> IIGG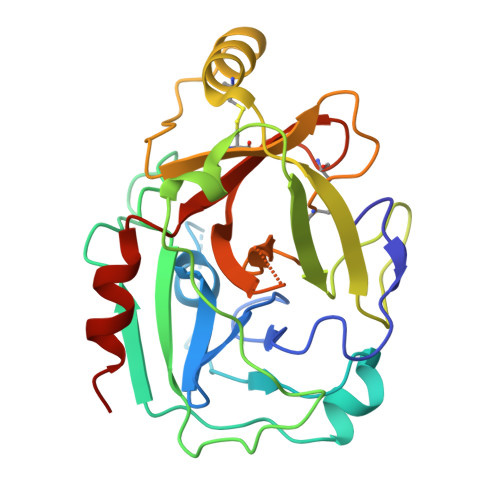QKAKMGNFPWQVFTNIHGRGGGALLGDRWILTAAHTLYPKEHEAQSNASLDVFLGHTNVEELMKLGNHPIRRVSVHPDYRQDESYNFEGDIALLELENSVTLGPNLLPICLPDNDTFYDLGLMGYVSGFGVMEEKIAHDLRFVRLPVANPQACENWLRGKNRMDVFSQNMFCAGHPSLKQDACQGDSGGVFAVRDPNTDRWVATGIVSWGIGCSRGYGFYTKVLNYVDWIKKEMEEED> MGYVEIIEQPKQRGMRFRYKCEGRSAGSIPGERSTDTTKTHPTIKINGYTGPGTVRISLVTKDPPHRPHPHELVGKDCRDGFYEAELCPDRCIHSFQNLGIQCVKKRDLEQAISQRIQTNNNPFQVPIEEQRGDYDLNAVRLCFQVTVRDP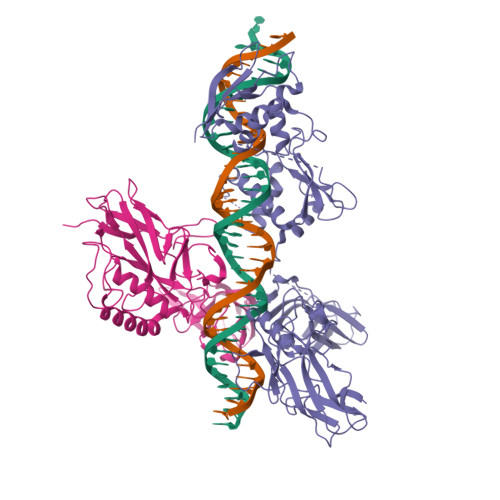SGRPLRLPPVLSHPIFDNRAPNTAELKICRVNRNSGSCLGGDEIFLLCDKVQKEDIEVYFTGPGWEARGSFSQADVHRQVAIVFRTPPYADPSLQAPVRVSMQLRRPSDRELSEPMEFQYLPDGSLSSGSSLSSPSAGAAPRVLFGEWLLGEISSGCYEGLQWLDEARTCFRVPWKHFARKDLSEADARIFKAWAVARGRWPPSSRGGGPPPEAETAERAGWKTNFRCALRSTRRFVMLRDNSGDPADQHKVYALSGSLSSDSSLSSPSALSPKPRILPWLVSQLDLGQLEGVAWVNKSRTRFRIPWKHGLRQDAQQEDFGIFQAWAEATGAYVPGRDKPDLPTWKRNFRSALNRKEGLRLAEDRSKDPHDPHKIYEFVNGLEHHHHHH;> MDGPYLQILEQPKQRGFRFRYVCEGPSHGGLPGASSEKNKKSYPQVKICNYVGPAKVIVQLVTNGKNIHLHAHSLVGKHCEDGICTVTAGPKDMVVGFANLGILHVTKKKVFETLEARMTEACIRGYNPGLLVHPDLAYLQAEGGGDRQLGDREKELIRQAALQQTKEMDLSVVRLMFTAFLPDSTGSFTRRLEPVVSDAIYDSKAPNASNLKIVRMDRTAGCVTGGEEIYLLCDKVQKDDIQIRFYEEEENGGVWEGFGDFSPTDVHRQFAIVFKTPKYKDINITKPASVFVQLRRKSDLETSEPKPFLYYPE>MAHSSATAGPQADYSGEIAELYDLVHQGKGKDYHREAADLAALVRRHSPKAASLLDVACGTGMHLRHLADSFGTVEGLEL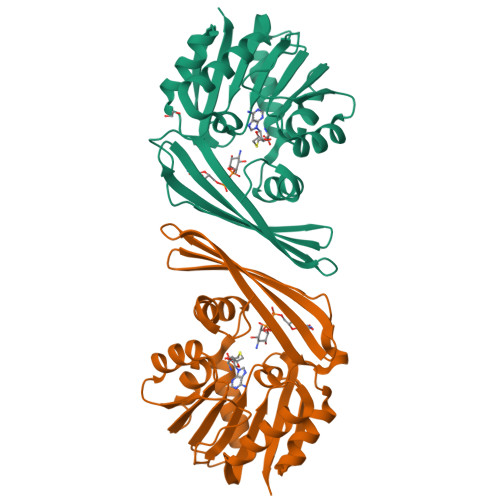SADMLAIARRRNPDAVLHHGDMRDFSLGRRFSAVTCMFSSIGALAGQAELDAALERFAAHVLPDGVVVVEPWWFPENFTPGYVAAGTVEAGGTTVTRVSHSSREGEATRIEVHYLVAGPDRGITHHEESHRITLFTREQYERAFTAAGLSVEFMPGGPSGRGLFTGLPGAKGETRLEHHHHHH[2x]>[2x]MMKPEDVIKEQCARAKVVAELWHGFTGGAPKAALENLVVEFNKAQQGRCVRPVPQGGYRDLSTKIKAAFAAGKVPTMAQAFENNIALYLEAKALLPIESLGVKLQGVNLTFLNAVRFGGVVYGVPFNKAIQVLYYNKDLLKKHGVPVPATLEEFVAAAKKLSR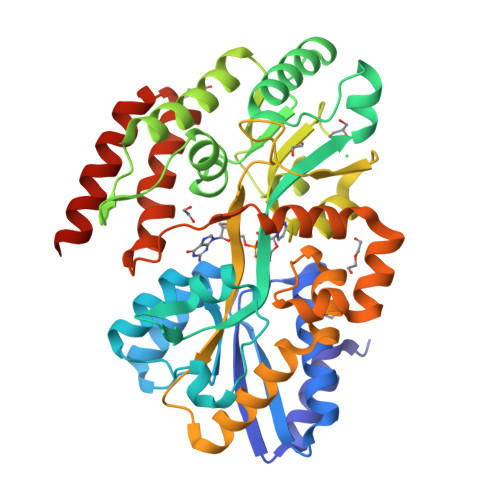AEGGPVYWFQPDASTFAYFFFNLGGSYLKDGKLVLNSKEAVEALTLLQNGVKEGWAKPITSGYINQNLGSGPYAFSVDTSAGYTYYLRAAKFDLGVATLPGRTKGQPGYGLVQGTNLVVFRQASKEEQAVAKDFLEFVLSPRAQAVFATATGYVPVTEGALKDPVYQAYAAENPDYATIVRQSRYAKFEPALAEWEQIRFDILGQAIKEAILNKADPKAALDRAQKLAEDLLSSRTRHHHHHH>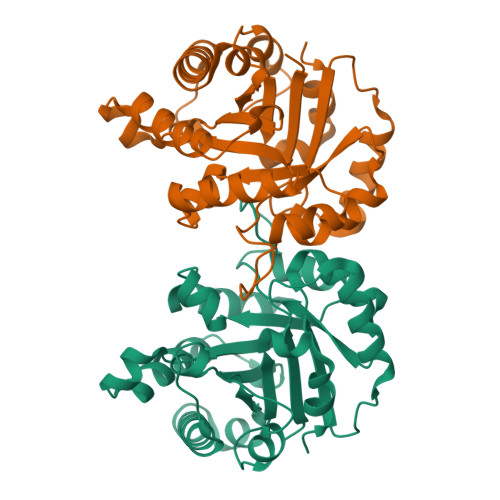[4x]MAPSRKFFVGGNWKMNGRKQSLGELIGTLNAAKVPADTEVVCAPPTAYIDFARQKLDPKIAVAAQNCYKVTNGAFTGEISPGMIKDCGATWVVLGHSERRHVFGESDELIGQKVAHALAEGLGVIACIGEKLDEREAGITEKVVFEQTKVIADNVKDWSKVVLAYEPVWAIGTGKTATPQQAQEVHEKLRGWLKSNVSDAVAQSTRIIYGGSVTGATCKELASQPDVDGFLMGGASLKPEFVDIINAKQ> YPPSMDWRKKGNFVSPVKNQGSCGSCWTFSTTGALESAVAIATGKMLSLAEQQLVDCAQNFNNHGCQGGLPSQAFEYIRYNKGIMGEDTYPYKGQDDHCKFQPDKAIAFVKDVANITMNDEEAMVEAVALYNPVSFAFEVTNDFLMYRKG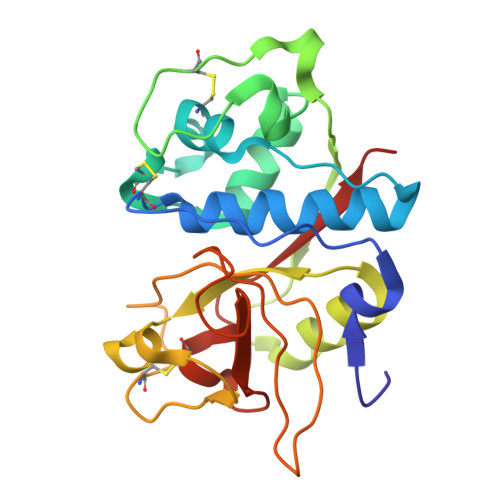IYSSTSCHKTPDKVNHAVLAVGYGEENGIPYWIVKNSWGPQWGMNGYFLIERGKNMCGLAACASYPIPLV>[2x]MSNPTKISILGRESIIADFGLWRNYVAKDLISDCSSTTYVLVTDTNIGSIYTPSFEEAFRKRAAEITPSPRLLIYNRPPGEV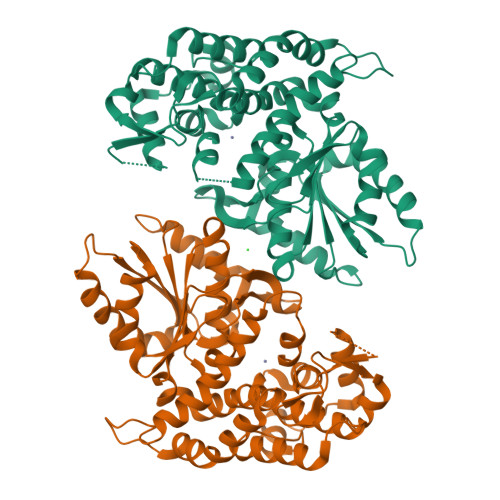SKSRQTKADIEDWMLSQNPPCGRDTVVIALGGGVIGDLTGFVASTYMRGVRYVQVPTTLLAMVDSSIGGKTAIDTPLGKNLIGAIWQPTKIYIDLEFLETLPVREFINGMAEVIKTAAISSEEEFTALEENAETILKAVRREVTPGEHRFEGTEEILKARILASARHKAYVVSADEREGGLRNLLNWGHSIGHAIEAILTPQILHGECVAIGMVKEAELARHLGILKGVAVSRIVKCLAAYGLPTSLKDARIRKLTAGKHCSVDQLMFNMALDKKNDGPKKKIVLLSAIGTPYETRASVVANEDIRVVLAP>[2x]TYLMNNYARLPVKFVRGKGVYLYDEEGKEYLDFVSGIGVNSLGHAYPKLTEALKEQVEKLLHVSNLYENPWQEELAHKLVKHFWTEGKVFFANSGTESVEAAIKLARKYWRDKGKNKWKFISFENSFHGRTYGSLSATGQPKFHKGFEPLVPGFSYAKLNDIDSVYKLLDEETAGIIIEVIQGEGGVNEASEDFLSKLQEICKEKDVLLIIDEVQTGIGRTGEFYAYQHFN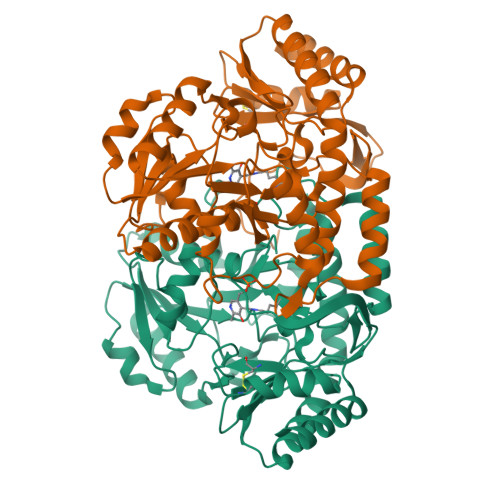LKPDVIALAKGLGGGVPIGAILAREEVAQSFTPGSHGSTFGGNPLACRAGTVVVDEVEKLLPHVREVGNYFKEKLKELGKGKVKGRGLMLGLELERECKDYVLKALEKGLLINCTAGKVLRFLPPLIIQKEHIDRAISVLREIL> NLFFPFTDAHKKLLNQMIRSNPKLMSGPFALLVKNQKVLDFDNKRYFFNAKLKSDNQERPKLPITVRREQVFLDSYRALFFKTNDEIKNSKLEITFKGESGVDAGGVTREWYQVLSRQMFNPDYALFLPVPSDKTTFHPNRTSALNPEHLSFFKFIGMIIGKAIRDQCFLDCHFSREVYKNILGRPVSLKDMESLDPDYYKSLVWILENDITDIIEETFSVETDDYGEHKVINLIEGGKDIIVTEANKQDYVKKVVEYKLQTSVKEQMDNFLVGFYALISKDLITIFDEQELELLISGLPDIDVDDWKNNTTYVNYTATCKEVSYFWRAVRSFDAEERAKLLQFVT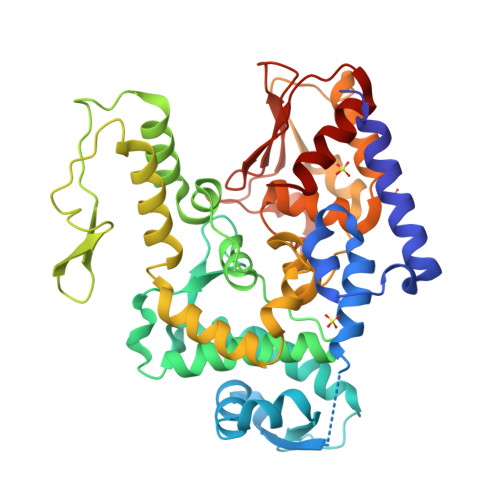GTSKVPLNGFKELSGVNGVCKFSIHRDFGSSERLPSSHTCFNQLNLPPYESYETLRGSLLLAINEG> 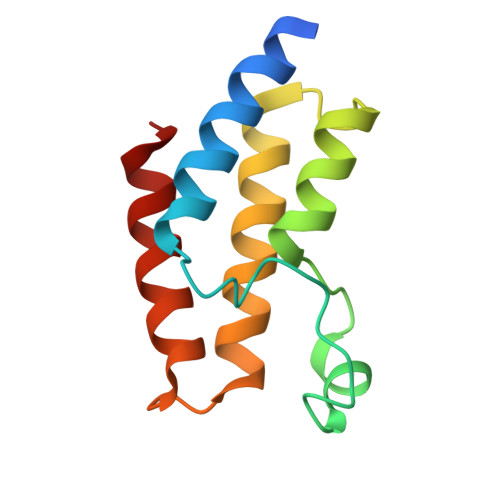GSAENESTPIQQLLEHFLRQLQRKDPHGFFAFPVTDAIAPGYSMIIKHPMDFGTMKDKIVANEYKSVTEFKADFKLMCDNAMTYNRPDTVYYKLAKKILHAGFKMMSK> MSDLQDQEPSIIINGNLEPVGEPDIVEETEVVAQETQETQDADKPKKKVAFTGLEEDGETEEEKRKREFEEGGGLPEQPLNPDFSKLNPLSAEIINRQATINIGTIGHVAHGKSTVVRAISGVQTVRFKDELERNITIKLGYANAKIYKCQEPTCPEPDCYRSFKSDKEISPKCQRPGCPGRYKLVRHVSFVDCPGHDILMSTMLSGAAVMDAALLLIAGNESCPQPQTSEHLAAIEIMKLKHVIILQNKVDLMREESALEHQKSILKFIRGTIADGAPIVPISAQLKYNIDAVNEFIVKTIPVPPRDFMISPRLIVIRSFDVNKPGAEIEDLKGGVAGGSILNGVFKLGDEIEIRPGIVTKDDKGKIQCKPIFSNIVSLFAEQNDLKFAVPGGLIGVGTKVDPTLCRADRLVGQVVGAKGHLPNIYTDIEINYFLLRRLLGVKTDGQKQAKVRKLEPNEVLMVNIGSTATGARVVAVKADMAR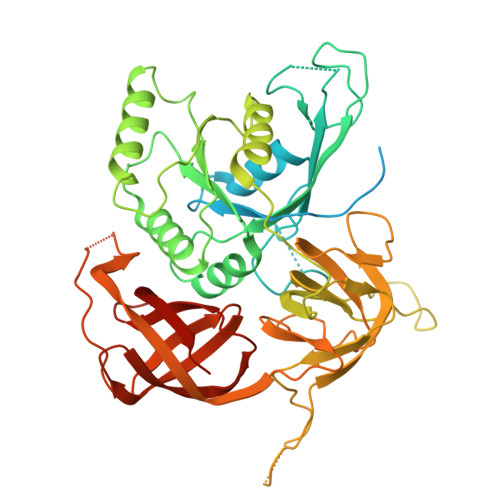LQLTSPACTEINEKIALSRRIEKHWRLIGWATIKKGTTLEPIA> KDSTGKCGPPPPIDNGGITSFPLSVYAPASSVEYQCANLYQLEGNKRITCRNGQWSEPPKCLHPCVISREIMENYNIALRWTAKQKLYSRTGESVEFVCKRGYR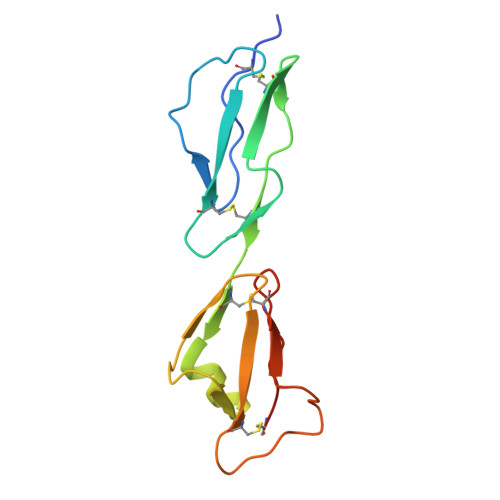LSSRSHTLRTTCWDGKLEYPTCAKR> MLESKLKAPVFTATTQGDHYGEFVLEPLERGFGVTLGNPLRRILLSSIPGTAVTSVYIEDVLHEFSTIPGVKEDVVEIILNLKELVVRFLDPRWRTTLILRAEGPKEVRAVDFTPSADVEIMNPDL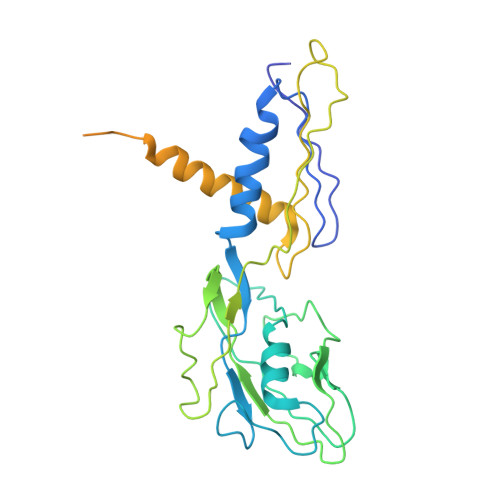HIATLEEGGKLYMEVRVDRGVGYVPAERHGIKDRINAIPVDAIFSPVRRVAFQVEDTRLGQRTDLDKLTLRIWTDGSVTPLEALNQAVAILKEHLNYFANPEASLLPTPEVSKGEKRESAEEDLDLPLEELGLSTRVLHSLKEEGIESVRALLALNLKDLRNIPGIGERSLEEIRQALAKKGFTLKE>[3x]AKLETVTLGNIGKDGKQTLVLNPRGVNP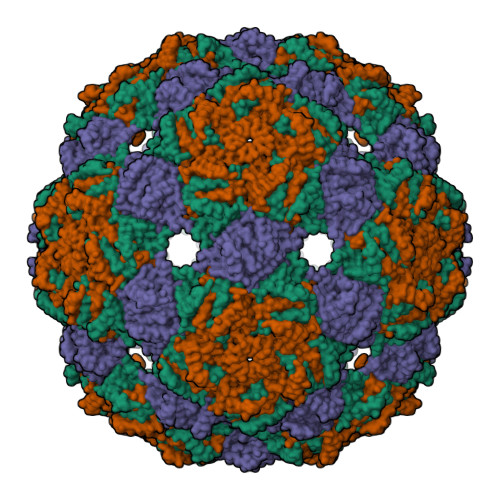TNGVASLSQAGAVPALEKRVTVSVSQPSRNRKNYKVQVKIQNPTACTANGSCDPSVTRQAYADVTFSFTQYSTDEERAFVRTELAALLASPLLIDAIDQLNPAY> MLESKLKAPVFTATTQGDHYGEFVLEPLERGFGVTLGNPLRRILLSSIPGTAVTSVYIEDVLHEFSTIPGVKEDVVEIILNLKELVVRFLDPKMASTTLILRAEGPKEVRAVDFTPSADVEIMNPDLHIATLEEGGKLYMEVRVDRGVGYVPAERHG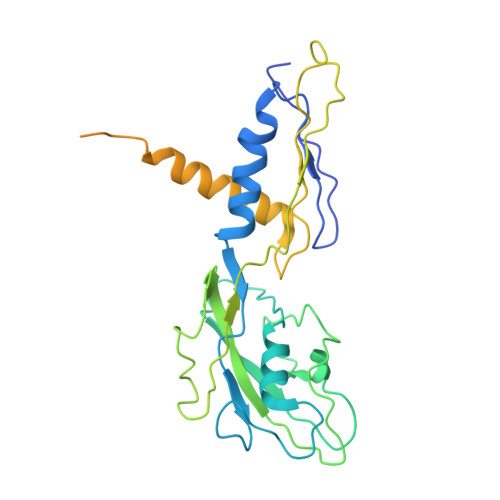IKDRINAIPVDAIFSPVRRVAFQVEDTRLGQRTDLDKLTLRIWTDGSVTPLEALNQAVAILKEHLNYFANPEASSLPTPEVSKGEKRESAEEDLDLPLEELGLSTRVLHSLKEEGIESVRALLALNLKDLRNIPGIGERSLEEIRQALAKKGFTLKE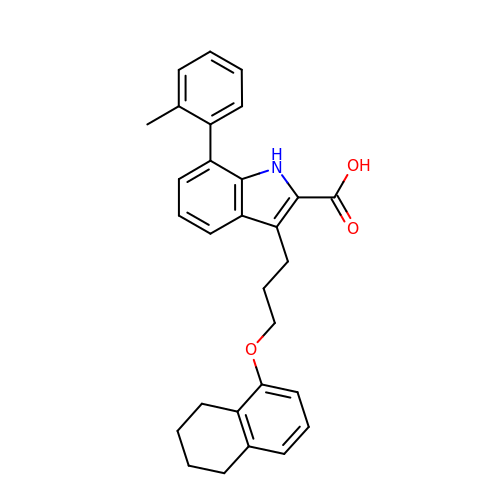7-(2-methylphenyl)-3-[3-(5,6,7,8-tetrahydronaphthalen-1-yloxy)propyl]-1~{H}-indole-2-carboxylic acid | C29 H29 N O3 | XMMADTDLICKLMQ-UHFFFAOYSA-N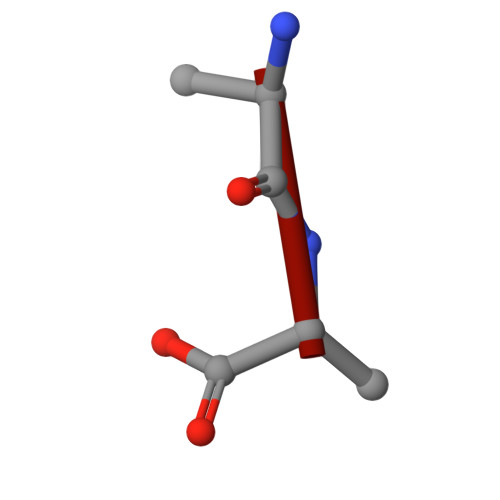> AA6-methoxy-streptovaricin C | C40 H53 N O14 | 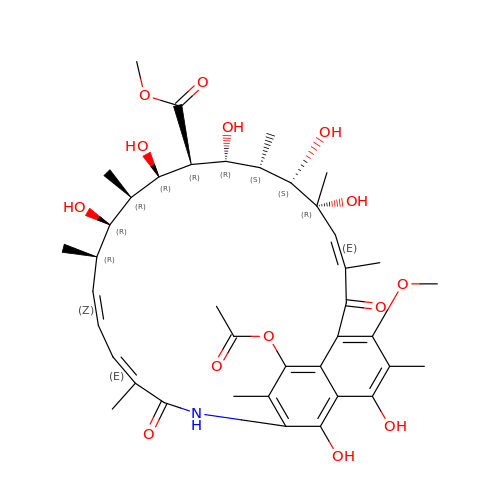KVBRXYBSUWPYTK-JYNZOJPESA-N> GMNNRELYGNIRDVYHLLQKNLDKAIEQYDISYVQFGVIQVLAKSGKVSMSKLIENMGCVPSNMT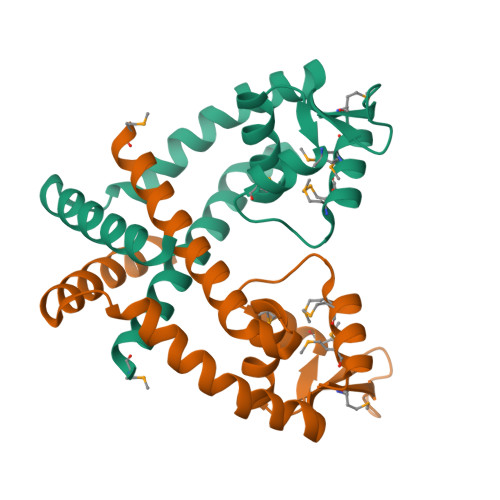TMIQRMKRDGYVMTEKNPNDQRETLVYLTKKGEETKKQVDVQYSDFLKENCGCFTKEEEGILEDLLLKWKKHLN>GSIINETADDIVYRLTVIIDDR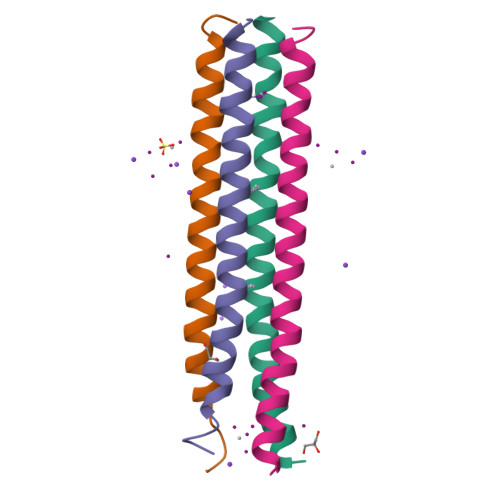YESLKNLITLRADRLEMIINDNVSTILASI[4x]>[5x]MVPTVQRGIIKMVLSGCAIIVRGQPRGGPPPERQINLSNIRAGNLARRAAATQPDAKDTPDEPWAFPAREFLRKKLIGKEVCFTIENKTPQGREYGMIYLGKDTNGENIAESLVAEGLATRREGMRANNPEQNRLSECEEQAKAAKKGMWSEGNGSHTIRDLKYTIENPRHFVDSHHQKPVNAIIEHVRDGSVVRALLLPDYYL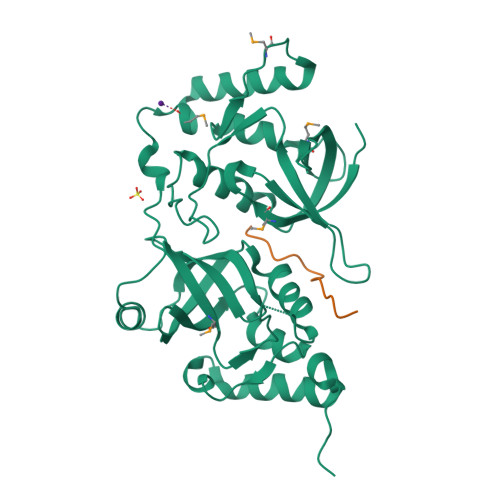VTVMLSGIKCPTFRREADGSETPEPFAAEAKFFTESRLLQRDVQIILESCHNQNILGTILHPNGNITELLLKEGFARCVDWSIAVYTRGAEKLRAAERFAKERRLRIWRDYVAPTANLDQK;>[5x]STGNASDSSSDSSSSEGDGTVSSADPNSDWNAPAEEWGNWVDE>[7x]MSIPVTEFRQFSEQQPAFRVLKPWWDVFTDYLSVAMLMIGVFGCTLQVMQDKIICLPKRVQPAQNHSSLSNVSQAVASTTPLPPPKPSPANPITVEMKGLKTDLDLQQYSFINQMCYERALHWYAKYFPYLVLIHTLVFMLCSNFWFKFPGSSSKIEHFISILGKCFDSPWTTRALSEVSGEDSEEKDNRKNNMNRSNTIQSGPEGSLVNSQSLKSIPEKFVVDKSTAGALDKKEGEQAKALFEKVKKFRLHVEEGDILYAMYVRQTVLKVIKFLIIIAYNSALVSKVQFTVDCNVDIQDMTGYKNFSCNHTMAHLFSKLSFCYLCFVSIYGLTCLYTLYWLFYRSLREYSFEYVRQETGIDDIPDVKNDFAFMLHMIDQYDPLYSKRFALFLSEVSENKLKQLNLNNEWTPDKLRQKLQTNAHNRLELPLIMLSGLPDTVFEITELQSLKLEIIKNVMIPATIAQLDNLQELSLHQCSVKIHSAALSFLKENLKVLSVKFDDMRELPPWMYGLRNLEELYLVGSLSHDISRNVTLESLRDLKSLKILSIKSNVSKIPQAVVDVSSHLQKMCIHNDGTKLVMLNNLKKMTNLTELELVHCDLERIPHAVFSLLSLQELDLKENNLKSIEEIVSFQHLRKLTVLKLWHNSITYIPEHIKKLTSLERLSFSHNKIEVLPSHLFLCNKIRYLDLSYNDIRFIPPEIGVLQSLQYFSITCNKVESLPDELYFCKKLKTLKIGKNSLSVLSPKIGNLLFLSYLDVKGNHFEILPPELGDCRALKRAGLVVEDALFETLPSDVREQMKADALEVLFQ

Volume-regulated anion channels (VRACs) constitute a diverse family of ion channels that are ubiquitously expressed in mammalian cells. They are believed to be essential for maintaining cellular volume, as they are known to open in response to hypotonic stress, enabling efflux of anions and osmolytes, thereby preventing excessive cell swelling and burst. VRACs are hexamers composed of five closely related paralogues of the leucine-rich repeat-containing protein 8 family (termed LRRC8A to E). In contrast, when expressed on its own, the LRRC8C subunit forms a larger, heptameric assembly with weaker mutual subunit interactions and a different preferential arrangement of the LRRDs.

The female patient carried a different monoallelic variant in LRRC8C, NM_032270.4:c.1168 G>C, p.(Val390Leu) (NC_000001.11:g.89713738 G>C [hg38], NC_000001.10:g.90179297 G>C [hg19]), or LRRC8CV390L, which also occurred in a de novo manner. In P1, the insertion of a base yields a frameshift in the amino acid sequence leading to a truncated protein, whereas the replacement of a valine by a leucine at position 390 leads to a moderate increase of the side chain volume without altering the hydrophobic character of the position. To investigate the biochemical properties of LRRC8C constructs carrying the disease variants, we compared the elution properties of overexpressed and purified WT and mutated human LRRC8C subunits as fusion to green fluorescent protein in HEK293 cells and found LRRC8CWT and LRRC8CV390L to elute as monodisperse peaks at the same volume, indicating that the presence of the point variant did not interfere with folding and oligomerization. Even though less pronounced than in LRRC8Ctrunc, related features in the map of LRRC8CV390L indicate a similarly increased subunit mobility. Akin to the truncated construct, also in case of the missense change, the ESD region is the best-defined part of the structure, obeying C7 symmetry and closely resembling WT. Despite the distinct difference between the two genetic variants, one (LRRC8CV390L) resulting in a conservative replacement of amino acid, the second (LRRC8Ctrunc) in the loss of an entire protein domain (representing ~50% of the protein), their structural and functional consequences are similar, leading to a strong increase of the subunit mobility in an oligomeric assembly and in consequence to a pronounced increase of activity even under isotonic conditions where VRACs are usually closed.> MHHHHHHMTSVMSHEFQLATAETWPNPWPMYRALRDHDPVHHVVPPQRPEYDYYVLSRHADVWSAARDHQTFSSAQGLTVNYGELEMIGLHDTPPMVMQDPPVHTEFRKLVSRGFTPRQVETVEPTVRKFVVERLEKLRANGGGDIVTELFKPLPSMVVAHYLGVPEEDWTQFDGWTQAIVAANAVDGATTGALD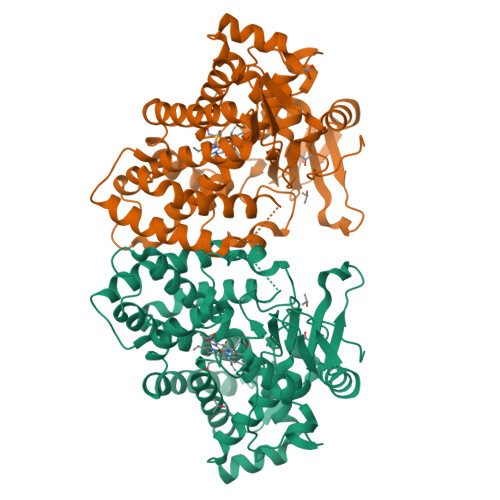AVGSMMAYFTGLIERRRTEPADDAISHLVAAGVGADGDTAGTLSILAFTFTMVTGGNDTVTGMLGGSMPLLHRRPDQRRLLLDDPEGIPDAVEELLRLTSPVQGLARTTTRDVTIGDTTIPAGRRVLLLYGSANRDERQYGPDAAELDVTRCPRNILTFSHGAHHCLGAAAARMQCRVALTELLARCPDFEVAESRIVWSGGSYVRRPLSVPFRVTSSR> MAAEEHALTSTEYIKHHLTNMTYGKMPDGTWKLAETAEEAHSMGFTAIHLDSMGWSIGLGVIFCLLFWIVARAANAGVPTKFQSAIEMIIEFVDSSVRDTFHGKSRLIAPLALTIFVWIFLMNLMDLIPVDWIPQVAAFVGANVFGMDPHHVYFKIVPSTDPNITLGMSLSVFVLILFYSIREKGVGGFVGELALNPFNPS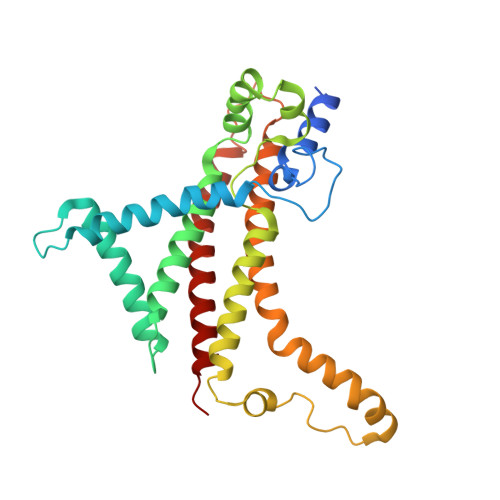NPVAKALLIPVNLILELVTFLARPISLALRLFGNMYAGELIFILIALLPFWIQWALSVPWAIFHILVITLQAFIFMMLTIVYLSMASEKH> MIDDDGYRPNVGIVISNRQGQVMWARRFGQHSWQFPQGGINPGESAEQAMYRELFEEVGLSRKDVRILASTRNWLRYKLPKRLVRWDTKPVCIGQKQKWFLLQLVSGDAEINMQTSSTPEFDGWRWVSYWYPVRQVVSFKRDVYRRVMKEFASV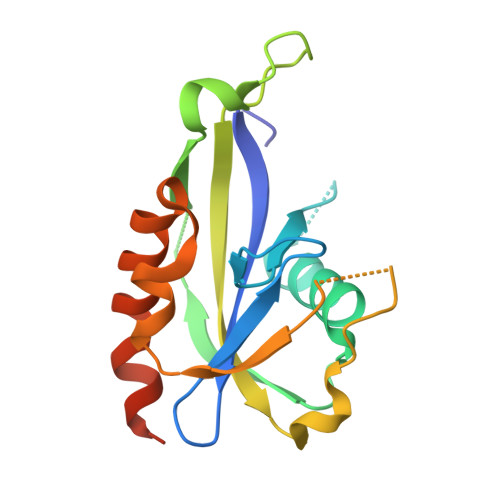VMSLLEHHHHHHHH PLLs are natural lactonases endowed with promiscuous phosphotriesterase activity. The catalytic center contained two metal cations coordinated by four histidines, an aspartic acid and a carboxylated lysine residue. A structural analysis of SsoPox, a hyperthermostable counterpart of the PLL family from Sulfolobus solfataricus, has revealed that loop 7 is shorter in SsoPox than in PTEs; linking the active site to the loop 8, which forms a hydrophobic channel that accommodates AHLs aliphatic chain. Indeed, W263 is located at the start of loop 8, involved in the dimer interface of the enzyme and positions the lactone cycle of the substrate onto the bi-metallic catalytic center.

Compared to wild-type SsoPox, variants W263L, W263M and W263F are the most efficient at improving specific activities, ranging from 30-50 and 20-35-fold at 1 mM and 100 µM, respectively. These variants constitute the Phosphotriesterase Selected Variants group (PteSV). Variant W263F is the most proficient (kcat/KM = 1.21 (±0.26)x104 M-1s-1), followed by W263M and W263L with increased efficiencies of 23.3, 14.1 and 4.6-fold, respectively, as compared to wild-type enzyme. The impact of this substitution is such that SsoPox-W263F hydrolyzes nerve agent analogs with remarkable efficiency (kcat/KM is 8.85 (±2.99)x104 M-1s-1 against IMP-coumarin), whereas the wild-type SsoPox is unable to hydrolyze this compound. The catalytic parameters obtained for CMP-coumarin (kcat/KM = 8.23 (±1.04)x104 M-1s-1), IMP-coumarin (kcat/KM = 8.85 (±2.99)x104 M-1s-1) and PinP-coumarin (kcat/KM = 7.08 (±2.58)x103 M-1s-1) hydrolysis enhanced catalytic efficiency 10- and 60-fold compared to the wild-type enzyme for which no activity was reported for PinP-coumarin. The variant W263F was also assayed in the presence of SDS, because anionic detergents have been shown to increase the phosphotriesterase activity of wild-type SsoPox. Interestingly, SDS has lower influence on the kinetic parameters of variant W263F against paraoxon and CMP-coumarin (with a catalytic efficiency increase ranging from 1.7 to 6.1-fold) than that observed for wild-type SsoPox (ranging from 6.4 to 12.4-fold). Thus, the W263F mutation might then mimic the SDS effect, by bringing local flexibility into the active site. Regarding the PteSV group, while these variants exhibit higher phosphotriesterase activity, they demonstrate mild improvements for the oxo-lactones and no or wild-type-like AHLase activity (W263L-M and W263F, respectively). The diffraction data for W263F and W263I-C10 HTL crystals were collected at the Proxima-1 beam line (SOLEIL, Gif-sur-Yvette, France) using a PILATUS-6M detector.

>[4x]MRIPLVGKDSIESKDIGFTLIHEHLRVFSEAVRQQWPHLYNEDEEFRNAVNEVKRAMQFGVKTIVDPTVMGLGRDIRFMEKVVKATGINLVAGTGIYIYIDLPFYFLNRSIDEIADLFIHDIKEGIQGTLNKAGFVKIAADEPGITKDVEKVIRAAAIANKETKVPIITHSNAHNNTGLEQQRILTEEGVDPGKILIGHLGDTDNIDYIKKIADKGSFIGLDRYGLDLFLPVDKRNETTLRLIKDGYSDKIMISHDYCCTIDFGTAKPEYKPKLAPRWSITLIFEDTIPFLKRNGVNEEVIATIFKENPKKFFS>MHHHHHHSSRENLYFQGQKESRACLERIQ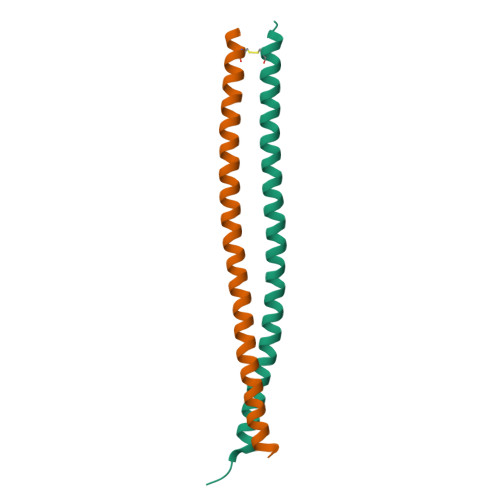ELEDLLAKEKDNSRRMLTDKEREMAEIRDQMQQQLNDYEQLLDVKLALDMEISAYRKLLEGEEERL[2x]>MSKVKVAVRVRPMNRREIDLHTKCVVDVEANKVILNPINTNLSKGDARGQPKIFAYDHCFWSMDESVREKCAGQDDVFKCLGENILQNAFDGYNACIFAYGQTGSGKSYTMMGTADQPGLIPRLCSGLFERTQKEENEEQSFKVEVSYMEIYNEKVRDLLDPKGSRQTLKVREHSVLGPY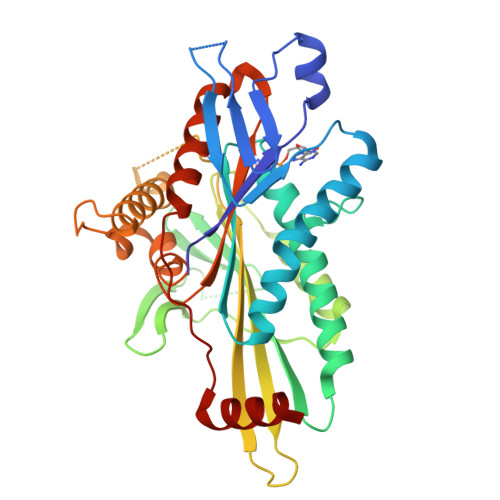VDGLSKLAVTSYKDIESLMSEGNKSRTVAATNMNEESSRSHAVFKITLTHTLYDVKSGTSGEKVGKLSLVDLAGSERATKTGAAGDRLKEGSNINKSLTTLGLVISALADQGAGKNKNKFVPYRDSVLTWLLKDSLGGNSKTAMVATVSPAADNYDETLSTLRYADRAKHIINHAVVNEDPNARIIRDLHHHHHH[3x]>[2x]MASQVSQMPSSSPLSSNKDEMRPKADFQPSIWGDLFLNCPDKNIDAETEKRHQQLKEEVRKMIVAPMANSTQKLAFIDSVQRLGVSYHFTKEIEDELENIYHNNNDAENDLYTTSIRFRLLREHGYNVSCDVFNKFKDEQGNFKSSVTSDVRGLLELYQASYLRVHGEDILDEAISFTTHHLSLAVASLDHPLSEEVSHALKQSIRRGLPRVEARHYLSVYQDIESHNKALLEFAKIDFNMLQFLHRKELSEICRWWKDLDFQRKLPYARDRVVEGYFWISGVYFEPQYSLGRKMLTKVIAMASIVDDTYDSYATYEELIPYTNAIERWDIKCIDEIPEYMKPSYKALLDVYEEMVQLVAEHGRQYRVEYAKNAMIRLAQSYLVEAKWTLQNYKPSFEEFKANALPTCG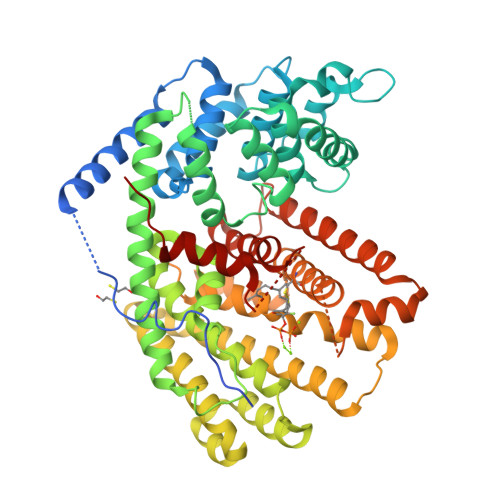YAMLAITSFVGMGDIVTPETFKWAASDPKIIQASTIICRFMDDVAEHKFKHRREDDCSAIECYMEEYGVTAQEAYDVFNKHVESAWKDLNQEFLKPTEMPTEVLNRSLNLARVMDVLYREGDGYTYVGKAAKGGITSLLIEPIAL> GLHSWGSEMDLVDSLDNPDEIQDNEEIQTQNVEAAQGEELATEVGLRATENDGSLSEQLNMSQPMFLNFKKHKVNIYAATHTKVDHIFGRAWAVGVFNTETAAIQKFDLHFPTSTHGALSRFFCHWTGELNIHILNVSTTNAFLKVAHTWFGTDSGIARTATLESNGTMIIPPNEQMTLCVPYYSEVPLRCVKGSDRNSAGLGSLFTQAVGRTISNRVQIFVSFRCPNFFFPLPAPREATSASILERVDEANAEELEAVLEARTPDAPLRLKFNPEDPLKQLREAAKAYFNIMHSDE;> MAASKMNPVGNLLSTVSSTVGSLLQNPSVEEKEMDSDRVAASTTTNAGNLVQASVAPTMPVKPDFKNTDDFLSMSYRSTTAPTNPTKMVHLAHGTWTTNQHRQALVASITLLQAFWPNQDFPAWGQSRYFAAVRCGFHIQVQLNVNIGSAGCLIAAYMPKTAHDHMNTYTFGSYTNLPHVLMNAATTSQADLYIPYVFNHNYARTDSDDLGGIYIWVWSALTVPSGSPTTVDVTIFGSLLDLDFQCPRPPGADTVIYTQ;> GKRTVRKTKTSKFKWVRNKIDIAEGPGAMNIANVLSTTGGQTIALVGERAFYDPRTAGAAVRCKDLMEIARMPSVFLGESTEPDGRRGYFTWSHTISPVNWVFDDHIYLENMPNLRLFSSCYN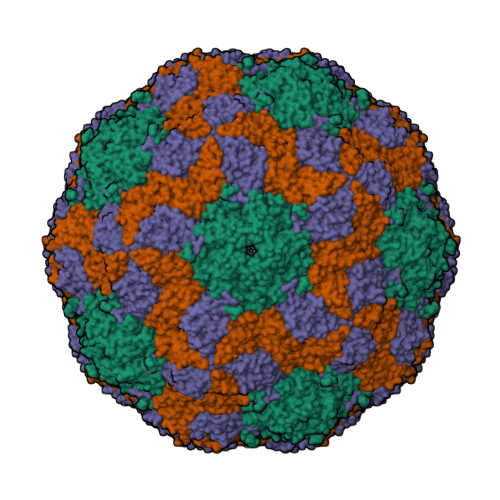YWRGSFVIKLTVYASTFNKGRLRMAFFPNREGAYTQDDAQNAIFVVCDIGLNNTFEMTIPYTWGNWMRPTRGNSLGHLRIDVLNRLTYNSSSPNAVNCILQIKMGDDAMFMVPTTSNLVMQ>MKTPRRRMRLAVFKALFQHEFRRDEDLEQILEEILDETYDKKAKEDARRYIRGIKE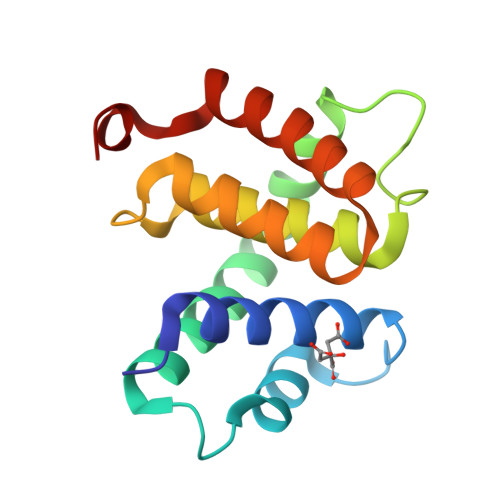NLSMIDDLISRYLEKWSLNRLSVVDRNVLRLATYELLFEKDIPIEVTIDEAIEIAKRYGTENSGKFVNGILDRIAKEHAPKEKFEL[2x]> GVPTCLLPGSNQFLTTDDHSSAPAFPDFSPTPEMHIPGQVHSMLEIVQIESMMEINNVNDASGVERLRVQISAQSDMDQLLFNIPLDIQLEGPLRNTLLGNISRYYTHWSGSLEMTFMFCGSFMTTGKLIICYTPPGGSSPTDRMQAMLATHVVWDFGLQSSITIIIPWISGSHYRMF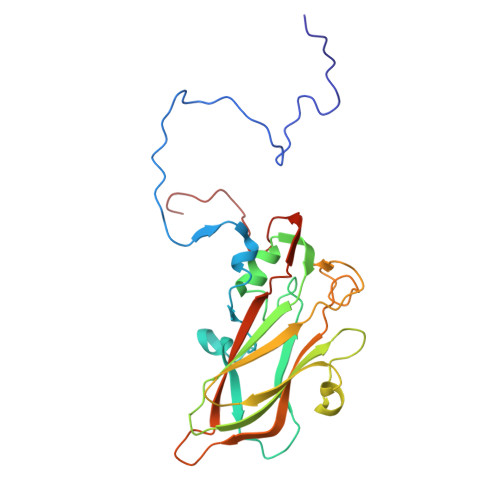NTDAKAINANVGYVTCFMQTNLVAPVGAADQCYIVGMVAAKKDFNLRLMRDSPDIGQSAILPEQA> GSHMIDKSAFVHPTAIVEEGASIGANAHIGPFCIVGPHVEIGEGTVLKSHVVVNGHTKIGRDNEIYQFASIGEVNQDLKYAGEPTRVEIGDRNRIRESVTIHRGTVQGGGLTKVGSDNLLMINAHIAHDCTVGNRCILANNATLAGHVSVDDFAIIGGMTAVHQFCIIGAHVMVGGCSGVAQDVPPYVIAQGNHATPFGVNIEGLKRRGFSREAITAIRNAY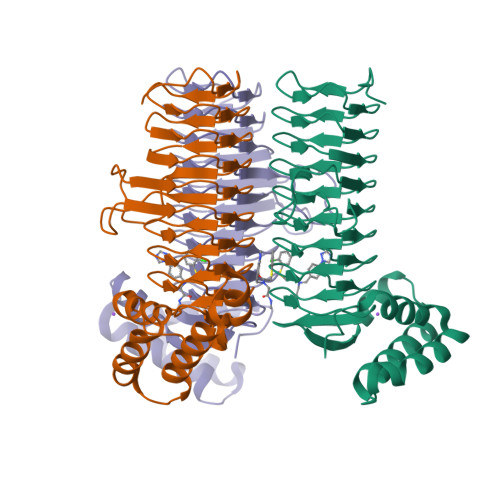KLIYRSGKTLDEVKPEIAELAETYPEVKAFTDFFARSTRGLIR>MARRLPKPTLQGRLEADFPDSPLLPKFQELNQNNLPNDVFREAQRSYLVFLTSQFCYEEYVQRTFGVPRRQRAIDKRQRASVAGAGAHAHLGGSSATPVQQAQAAASAGTGALASSAPSTAVAQSATPSVSSSISSLRAATSGATAAASAAAAVDTGSGGGGQPHDTAPRGARKKQ[16x];>MKVQGSVDRRRLQRRIAGLLPPPARRLNISRGSEFTRDVRGLVEEHAQASSLSAAAVWRAGLLAPGEVAVAGGGSGGGSFSWSGWRPPVFGDFLIHASSFNNAEATGTPLFQFKQSDPFSGVDAVFTPLSLFILMNHGRGVAARVEAGGGLTRMANLLYDSPATLADLVPDFGRLVADRRFHNFITPVGPLVENIKSTYLNKITTVVHGPVVSKAIPRSTVKVTVPQEAFVDLDAWLSGGAGGGGGVCFVGGLGLQPCPADARLYVALTYEEAGPRFTFFQSSRGHCQIMNILRIYYSPSIMHRYAVVQPLHIEELTFGAVACLGTFSATDGWRRSAFNYRGSSLPVVEIDSFYSNVSDWEVIL[5x];>[10x]MDLKVVVSLSSRLYTDEIAKMQQRIGCILPLASTHGTQNVQGLGLGQVYSLETVPDYVSMYNYLSDCTLAVLDEVSVDSLILTKIVPGQTYAIKNKYQPFFQWHGTGSLSVMPPVFGREHATVKLESNDVDIVFPMVLPTPIAEEVLQKILLFNVYSRVVMQAPGNADMLDVHMHLGSVSYLGHHYELALPEVPGPLGLALLDNLSLYFCIMVTLLPRASMRLVRGLIRHEHHDLLNLFQEMVPDEIARIDLDDLSVADDLSRMRVMMTYLQSLASLFNLGPRLATAAYSQETLTATCWLR;>MASNEGVENRPFPYLTVDADLLSNLRQSAAEGLFHSFDLLVGKDAREAGIKFEVLLGVYTNAIQYVRFLETALAVSCVNTEFKDLSRMTDGKIQFRISVPTIAHGDGRRPSKQRTFIVVKNCHKHHISTEMELSMLDLEILHSIPETPVEYAEYVGAVKTVASALQFGVDALERGLINTVLSVKLRHAPPMFILQTLADPTFTERGFSKTVKSDLIAMFKRHLLEHSFFLDRAENMGSGFSQYVRSRLSEMVAAVSGESVLKGVSTYTTAKGGEPVGGVFIVTDNVLRQLLTFLGEEADNQIMGPSSYASFVVRGENLVTAVSYGRVMRTFEHFMARIVDSPEKAGSTKSDLPAVAAGVEDQPRVPISAAVIKLGNHAVAVESLQKMYNDTQSPYPLNRRMQYSYYFPVGLFMPNPKYTTSAAIKMLDNPTQQLPVEAWIVNKNNLLLAFNLQNALKVLCHPRLHTPAHTLNSLNAAPAPRDRRETYSLQHRRPNHMNVLVIVDEFYDNKYAAPVTDIALKCGLPTEDFLHPSNYDLLRLELHPLYDIYIGRDAGERARHRAVHRLMVGNLPTPLAPAAFQEARGQQFETATSLAHVVDQAVIETVQDTAYDTAYPAFFYVVEAMIHGFEEKFVMNVPLVSLCINTYWERSGRLAFVNSFSMIKFICRHLGNNAISKEAYSMYRKIYGELIALEQALMRLAGSDVVGDESVGQYVCALLDPNLLPPVAYTDIFTHLLTVSDRAPQIIIGNEVYADTLAAPQFIERVGNMDEMAAQFVALYGYRVNGDHDHDFRLHLGPYVDEGHADVLEKIFYYVFLPTCTNAHMCGLGVDFQHVAQTLAYNGPAFSHHFTRDEDILDNLENGTLRDLLEISDLRPTVGMIRDLSASFMTCPTFTRAVRVSVDNDVTQQLAPNPADKRTEQTVLVNGLVAFAFSERTRAVTQCLFHAIPFHMFYGDPRVAATMHQDVATFVMRNPQQRAVEAFNRPEQLFAEYREWHRSPMGKYAAECLPSLVSISGMTAMHIKMSPMAYIAQAKLKIHPGVAMTVVRTDEILSENILFSSRASTSMFIGTPNVSRREARVDAVTFEVHHEMASIDTGLSYSSTMTPARVAAITTDMGIHTQDFFSVFPAEAFGNQQVNDYIKAKVGAQRNGTLLRDPRTYLAGMTNVNGAPGLCHGQQATCEIIVTPVTADVAYFQKSNSPRGRAACVVSCEN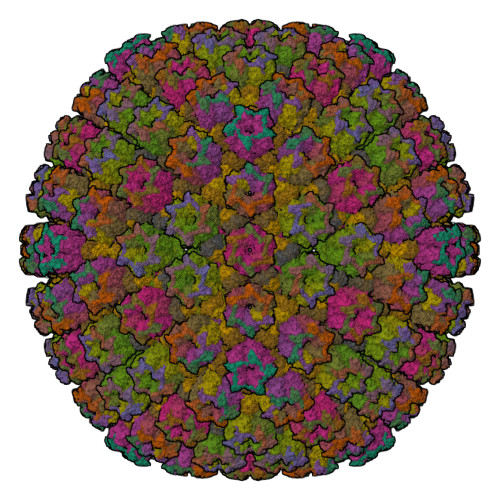YNQEVAEGLIYDHSRPDAAYEYRSTVNPWASQLGSLGDIMYNSSYRQTAVPGLYSPCRAFFNKEELLRNNRGLYNMVNEYSQRLGGHPATSNTEVQFVVIAGTDVFLEQPCSFLQEAFPALSASSRALIDEFMSVKQTHAPIHYGHYIIEEVAPVRRILKFGNKVVF[16x]> MNVRLCYASQRNEKNEDLL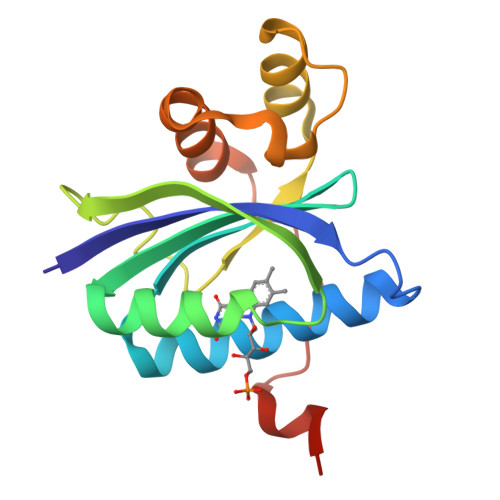QDLRDILTEARDFNDLNGICGVLYYADNAFFQCLEGEQEVVERLFEKIQKDQRHYNIKWLCTYSIDEHSFQRWSMKYVQRNTNIETFFLNMGENTFNPLLLNQQNLKFFLNELLIAEQTKMNTVKKVGMVNRGVNPF> GSSHHHHHHSQDLENLYFQGSQETLVRPKPLLLKLLKSVG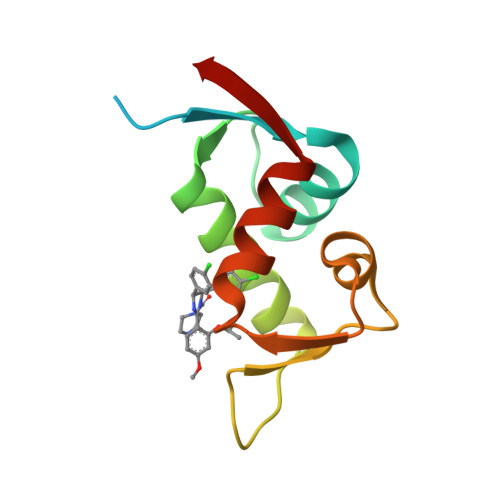AQKDTYTMKEVLFYLGQYIMTKRLYDEKQQHIVYCSNDLLGDLFGVPSFSVKEHRKIYTMIYRNLVVVNQ>VTQALVKEEIQAKEYLENLNKELAKRTNVETEAAWAYRSAITDENEKKKNEISAELAKFMKEVASDTTKFQWRSYQSEDLKRQFKALTKLGYAALPEDDYAELLDTLSAMESNFAKVKVCDYKDSTKCDLALDPEIEEVISKSRDHEELAYYWREFYDKAGTAVRSQFERYVELNTKAAK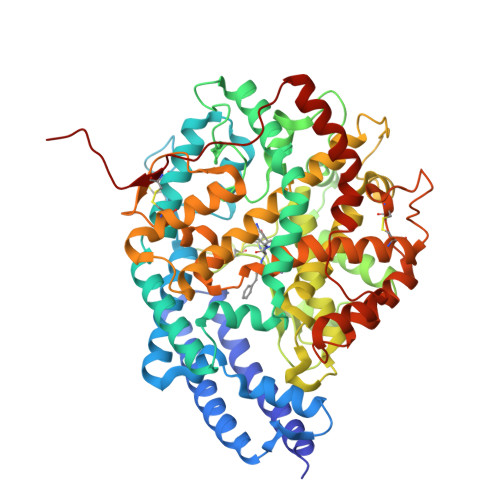LNNFTSGAEAWLDEYEDDTFEQQLEDIFADIRPLYQQIHGYVRFRLRKHYGDAVVSETGPIPMHLLGNMWAQQWSEIADIVSPFPEKPLVDVSAEMEKQAYTPLKMFQMGDDFFTSMNLTKLPQDFWDKSIIEKPTDGRDLVCHASAWDFYLIDDVRIKQCTRVTQDQLFTVHHELGHIQYFLQYQHQPFVYRTGANPGFHEAVGDVLSLSVSTPKHLEKIGLLKDYVRDDEARINQLFLTALDKIVFLPFAFTMDKYRWSLFRGEVDKANWNCAFWKLRDEYSGIEPPVVRSEKDFDAPAKYHISADVEYLRYLVSFIIQFQFYKSACIKAGQYDPDNVELPLDNCDIYGSARAGAAFHNMLSMGASKPWPDALEAFNGERIMSGKAIAEYFEPLRVWLEAENIKNNVHIGWITSNKCVSSHHHHH[2x]>MEFYNSTNEIPEEMLKGIDLTYPQLTYLPETGILYDNTYNEKTVPIISGGGSGHEPAHVGYVGSGMLAAAVTGPLFIPPKSKNILKAIRQVNSGKGVFVIIKNFEADLKEFNEAIKEARTEGIDVRYIVSHDDISVNAYNFHKRHRGVAGTILLHKILGAFAKEGGSIDEIEQLALSLSPEIYTLGVALAP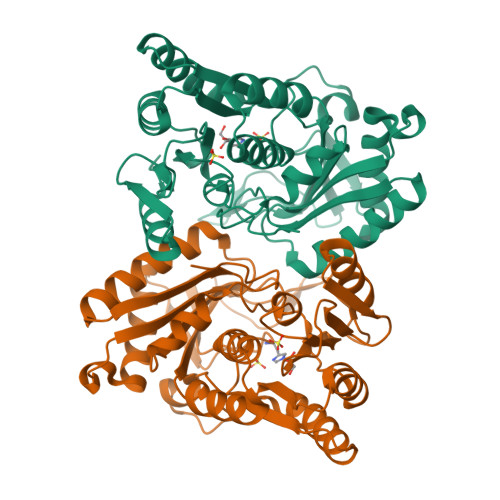VHFPHQKTSFVLAEDEVSFGIGIHGEPGYRVEKFEGSERIAIELVNKLKAEINWQKKANKNYILLVNGLGSTTLMELYSFQYDVMRLLELEGLSVKFCKVGNLMTSCDMSGISLTLCSVKDPKWLDYLNVPTGAFAWLEHHHHHH[2x]>[4x]MRIVPFGAAREVTGSAHLLLAGGRRVLLDCGMFQGKEEARNHAPFGFDPKEVDAVLLTHAHLDHVGRLPKLFREGYRGPVYATRATVLLMEIVLEDALKVMDEPFFGPEDVEEA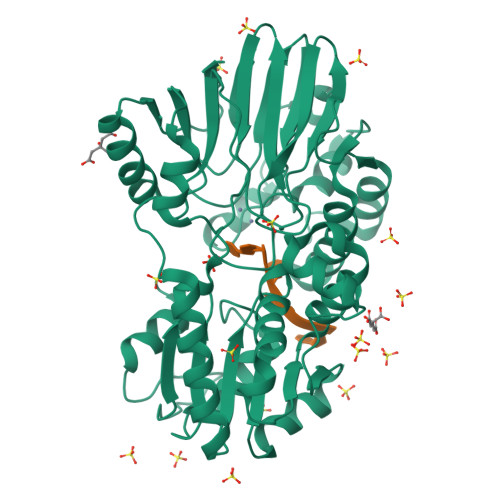LGHLRPLEYGEWLRLGALSLAFGQAGHLPGSAFVVAQGEGRTLVYSGDLGNREKDVLPDPSLPPLADLVLAEGTYGDRPHRPYRETVREFLEILEKTLSQGGKVLIPTFAVERAQEILYVLYTHGHRLPRAPIYLDSPMAGRVLSLYPRLVRYFSEEVQAHFLQGKNPFRPAGLEVVEHTEASKALNRAPGPMVVLAGSGMLAGGRILHHLKHGLSDPRNALVFVGYQPQGGLGAEIIARPPAVRILGEEVPLRASVHTLGGFSGAAGQDELLDWLQGEPRVVLVHGEEEKLLALGKLLALRGQEVSLARFGEGVPV> MDWEKVGLKMGLEIHQQLDTESKLFCPCRTELTDSEPDHDIVRNLRPTQSELGKFDRAAFEEAMRKLHFHYENYHEETCLVEADEEPPHPLNPEALEIAVTIALLLNMRVVDEFHTMRKQVIDGSNTGGFQRTGLVATDGHLETPQGTVKIENLCLEEDAARRIRETGDGVVFRLDRLGIPLVEITTDPSMSDPQQLREVAYQIGQILRSTRVKRGLGTIRQDLNISIRDGARVEVKGVQDLDLIPEIVEREVKRQLSLVEIRDTLQERGAVVEDKIFDVSEVFADTESRIISSAESVLAVKLRGFDGLIGVEIQPGRRLGTEMADYAKKRGVSGIFHTDELPAYGITEEEVRGLRDAVGASQGDAVVMVAHERVTAENALREVIRRAEMAIQGVPEETRKALPDGNTQYLRPLPTSSRMYLETDIPLFRIEDDLLEG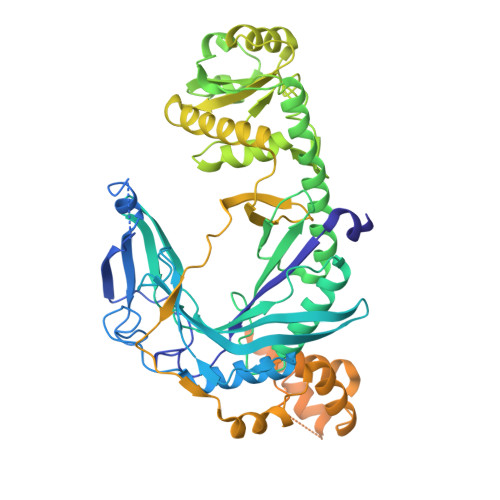IRRNLPELPSEKKERIMRDYGLSEDLASQLVKRNLVDEFEALTEFRVDTTVIASLLAYTLRELRREGHDVDGLGLDELRDAIKLLEVGKISKDALRDIVACMADEGLAAEDAARKLNLLLLAEDEIESIIQEIVEGNLDMISERGMGAMGPLMGQAMGRLRGRADGKVVNRILREKIQERL>[2x]MNKLHKGWFTEFSPDDLEKMNGASDEEPTKVLKSDGQEMGGAWPGQAFSLQVKKVLFHEKSKYQDVLVFESTTYGNVLVLDGIVQATERDEFSYQEMLAHLPMFAHPDPKRVLIIGGGDGGILREVLKHESVEKVTMCEIDEMVIDVAKKFLPGMSCGFSHPKLDLFCGDGFEFLKNHKNEFDVIITD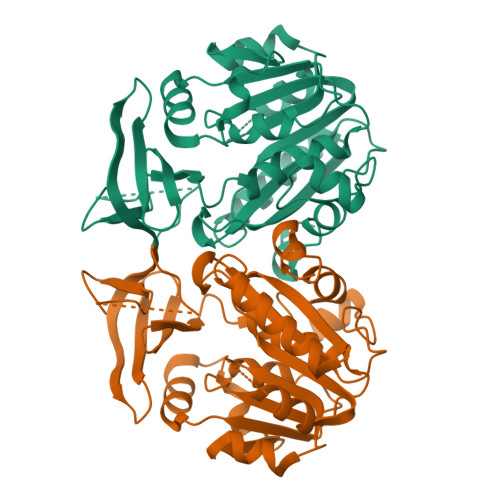SSDPVGPAESLFGQSYYELLRDALKEDGILSSQGESVWLHLPLIAHLVAFNRKIFPAVTYAQSIVSTYPSGSMGYLICAKNANRDVTTPARTLTAEQIKALNLRFYNSEVHKAAFVLPQFVKNALE(S)-2-({4-[3-(2-Amino-4-oxo-4,7-dihydro-3H-pyrrolo[2,3-d]pyrimidin-6-yl)-propyl]-thiophene-2-carbonyl}-amino)-pentanedioic 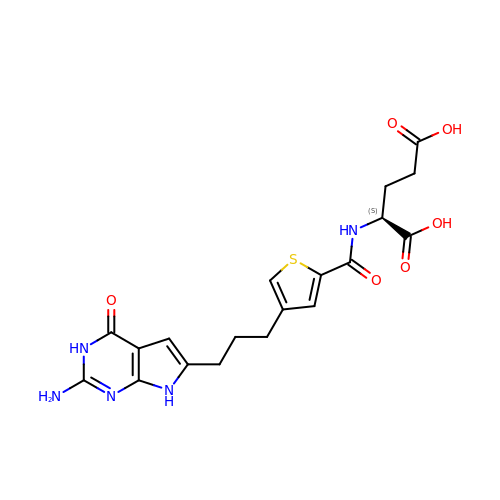acid | C19 H21 N5 O6 S | UNSSSMUKJOLMJV-LBPRGKRZSA-N> XWIAQ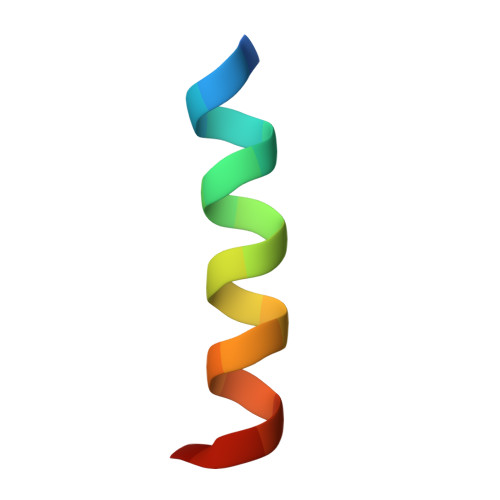ELREIGDKFNAYYAX> MLRDLFDRAVVLSAYIHNLSSEMFSEFDKRYTHGRGFITKAINSCHTSSLATPEDKEQAQQMNQKDFLSLIVSILRSWNEPLYHLVTEVRGMQEAPEAILSKAVEIEEQTKRLLER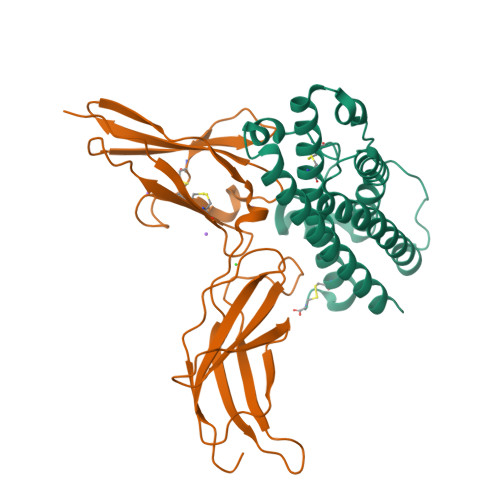MELIVSQVHPETKENEIYPVWSGLPSLQMADEESRLSAYYNLLHCLRRDSHKIDNYLKLLKCRIIHNNNC;> MLPPGKPEIFKCRSPNKETFTCWWRPGTDGGLPTNYSLTYHREGETLMHECPDYITGGPNSCHFGKQYTSMWRTYIMMVNATNQMGSSFSDELYVDVTYIVQPDPPLELAVEVKQPEDRKPYLWIKWSPPTLIDLKTGWFTLLYEIRLKPEKAAEWEIHFAGQQTEFKILSLHPGQKYLVQVRCKPDHGYWSAWSPATFIQIPSDFTMND> MGSSHHHHHHSQDLEVLFQGPGSMEDAKNIKKGPAPFYPLEDGTAGEQLHKAMKRYALVPGTIAFTDAHIEVNITYAEYFEMSVRLAEAMKRYGLNTNHRIVVCSENSLQFFMPVLGALFIGVAVAPANDIYNERELLNSMNISQPTVVFVSKKGLQKILNVQKKLPIIQKIIIMDSKTDYQGFQSMYTFVTSHLPPGFNEYDFVPESFDRDKTIALIMNSSGSTGLPKGVALPHRTACVRFSHARDPIFGNQIIPDTAILSVVPFHHGFGMFTTLGYLICGFRVVLMYRFEEELFLRSLQDYKIQSALL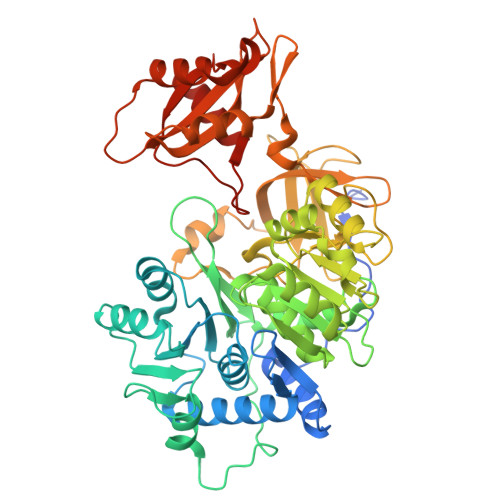VPTLFSFFAKSTLIDKYDLSNLHEIASGGAPLSKEVGEAVAKRFHLPGIRQGYGLTETTSAILITPEGDDKPGAVGKVVPFFEAKVVDLDTGKTLGVNQRGELCVRGPMIMSGYVNNPEATNALIDKDGWLHSGDIAYWDEDEHFFIVDRLKSLIKYKGYQVAPAELESILLQHPNIFDAGVAGLPDDDAGELPAAVVVLEHGKTMTEKEIVDYVASQVTTAKKLRGGVVFVDEVPKGLTGKLDARKIREILIKAKKGGKSKL>HGSSHHHHHHSSENLYFQGHMWNSRKVGVLGGGQLGRMLVESANRLNIQVNVLDADNSPAKQISAHDGHVTGSFKEREAVRQLAKTCDVVTAEIEHVDTYALEEVASEVKIEPSWQAIRTIQNKFNQKEHLRKYGIPMAEHRELVENTPAELAKVGEQLGYPLMLKSKTMAYDGRGNFRVNSQDDIPEALEALKDRPLYAEKWAYFKMELAVIVVKTKDEVLSYPTVETVQEDSICKLVYAPARNVSDAINQKAQELARKAVAAFDGKGVFGVEMFLLEDDSIMLCEIASRIHNSGHYTIEGCALSQFDAHLRAILDLPIPAQSLEIRQPSIMLNIIGGAA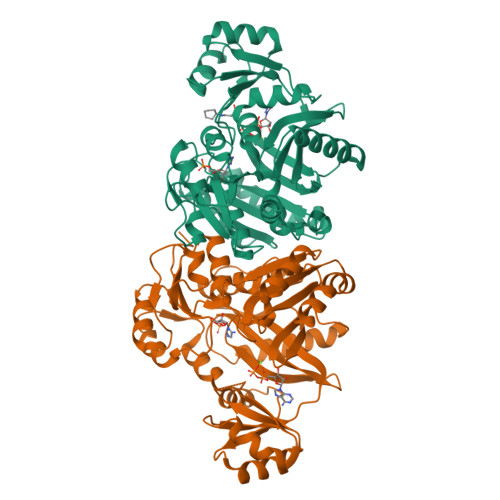PDTHLQAAECALSIPNASIHLYSKGAAKPGRKMGHITVTAPTMHEAETHIQPLIDVVDRIRA[4x]>[4x]CCGG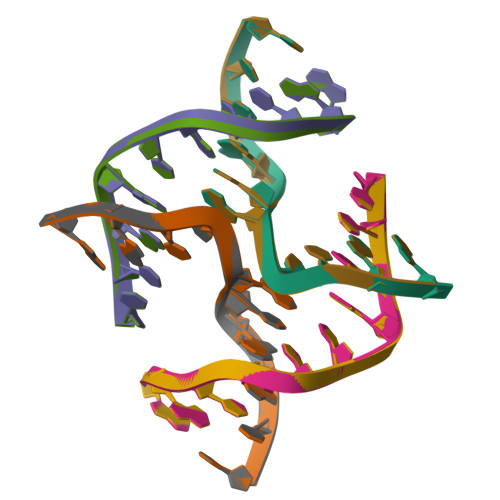TANCGG;>CCGATACCGG[4x]>MRGSHHHHHHGMASMPLHHLTRFPRLEFIGAPTPLEYLPRLSDYLGREIYIKRDDVTPIAMGGNKLRKLEFLVADALREGADTLITAGAIQSNHVRQTAAVAAKLGLHCVALLENPIGTTAENYLTNGNRLLLDLFNTQIEMCDALTDPDAQLQTLATRIEAQGFRPYVIPVGGSSALGAMGYVESALEIAQQCEEVVGLSSVVVASGSAGTHAGLAVGLEHLMPDVELIGVTVSR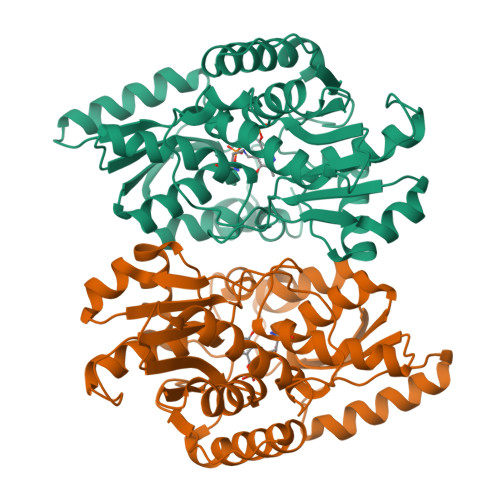SVAEQKPKVIALQQAIAGQLALTATADIHLWDDYFAPGYGVPNDAGMEAVKLLASLEGVLLDPVYTGKAMAGLIDGISQKRFNDDGPILFIHTGGAPALFAYHPHV[8x]The TNA backbone is composed of phosphodiester-linked 3′→2′ α-l-threofuranose sugars and, therefore, has one fewer atom in its repeating unit than RNA. Critically, TNA can form stable Watson−Crick duplexes with itself, DNA and RNA, such that the exchange of genetic information between these polymers appears feasible. Here, we examine the behaviour of TNA in nonenzymatic template-directed primer extension reactions from both a kinetic and a structural perspective. Taken together, we propose that structural constraints explain the diminished ability of TNA to engage in nonenzymatic template-directed primer extension, and we discuss the consequences of these observations for the plausibility of the involvement of TNA in the origin of primitive cells.

Here, we carried out a similar procedure by soaking the same RNA-dGMP co-crystals with a solution of the activated threo-nucleotide monomer 2AIptG. The optimal structure was determined after soaking the RNA-dGMP crystal in a 20 mM 2AIptG solution for 24 h. At each end of the A-helical duplex, we observe density consistent with imidazolium-bridged TNA guanosine dinucleotides (tGp-AI-ptG) bound to the template (TNA-D1). It is noteworthy that formation of the tGp-AI-ptG intermediate in the crystal was much slower than formation of the corresponding RNA intermediate Gp-AI-pG (24 h versus ∼1 h), consistent with our solution phase NMR observations. Critically, the electron density between the two nucleotides is consistent with the formation of an imidazolium bridge. The distance between the 3′-OH of the primer and the incoming P atom of tGp-AI-ptG molecule is ∼5.9 Å in the refined model. This distance is significantly longer than that observed in the RNA complex containing native Gp-AI-pG (4.6 Å). Furthermore the O-P-N angle of attack is 122°, which is less than the previously observed angles of 132° and 170° for the all-RNA complex. Both the longer distance and smaller angle could contribute to the slower primer extension observed with activated threo-nucleotides.

>[2x]NNNGACUUAAGUCG6S,6aS,7R,10S,10aR)-6-(3,5-bis(trifluoromethyl)phenyl)-5,6,6a,7,8,9,10,10a-octahydro-7,10-methanophenanthridine-3-carboxylic acid 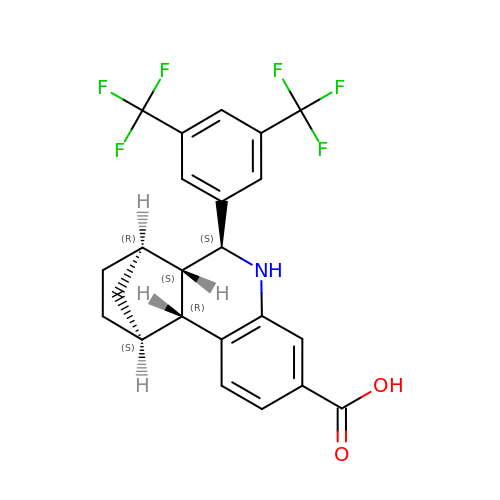| C23 H19 F6 N O2 | GGGBDYORXLHJAW-QRHYTPHYSA-N> MFEARLVQGSILKKVLEALKDLINEACWDISSSGVNLQSMDSSHVSLVQLTLRS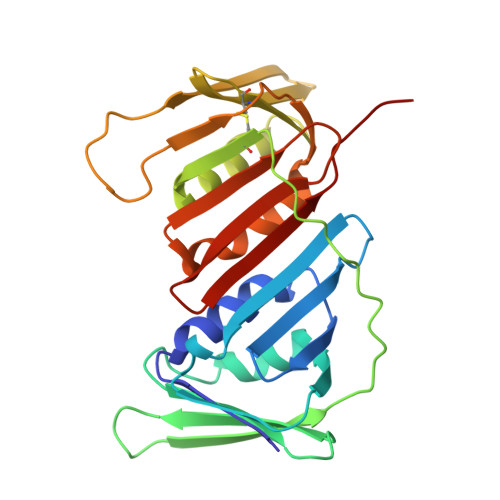EGFDTYRCDRNLAMGVNLTSMSKILKCAGNEDIITLRAEDNADTLALVFEAPNQEKVSDYEMKLMDLDVEQLGIPEQEYSCVVKMPSGEFARICRDLSHIGDAVVISCAKDGVKFSASGELGNGNIKLSQTSNVDKEEEAVTIEMNEPVQLTFALRYLNFFTKATPLSSTVTLSMSADVPLVVEYKIADMGHLKYYLAPKIEDE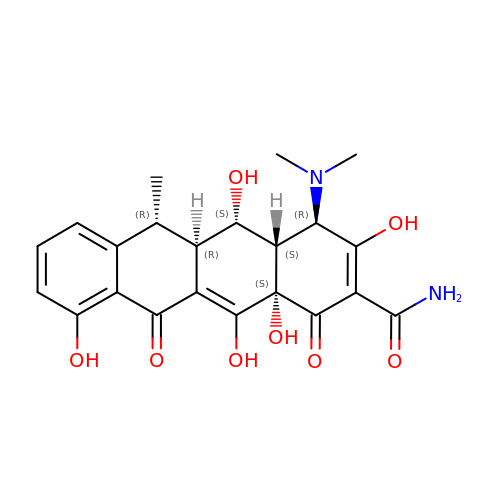(4S,4AR,5S,5AR,6R,12AS)-4-(DIMETHYLAMINO)-3,5,10,12,12A-PENTAHYDROXY-6-METHYL-1,11-DIOXO-1,4,4A,5,5A,6,11,12A-OCTAHYDROTETRACENE-2-CARBOXAMIDE | C22 H24 N2 O8 | JBIWCJUYHHGXTC-AKNGSSGZSA-N> GHMDEISETNTIFKLEGVSVLSPLRKKLDLVFYLSNVDGSPVITLLKGNDRELSIYQLNKNIKMASFLPVPEKPNLIYLFMTYTSCEDNKFSEPVVMTLNKENTLNQFKKLGLLDSNVTDFEKCVEYIRKQAILTGFKISNPFVNSTLVDTDAEKINSFHLQCHRGTKEGTLYFLPDHIIFGFKKPILLFDASDIESITYSSITRLTFNASLVTKDGEKYEFSMIDQTEYAKIDDYVKRK;> MRDSTECQRIIRRGVNCLMLPKGMQRSSQNRSKWDKTMDLFVWSVEWILCPMQEKGEKKELFKHVSHRIKETDFLVQGMGKNVFQKCCEFYRLAGTSSCIEGEDGSETKEERTQILQKSGLKFYTKTFPYNTTHIMDSKKLVELAIHEKCIGELL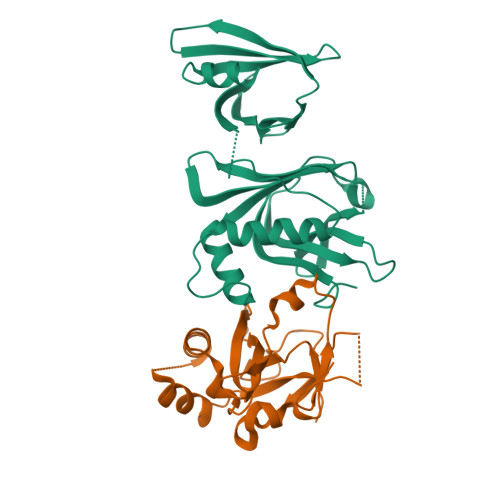KNTTVIEFPTIFVAMTEADLPEGYEVLHQE> SYFEPTGPYLMVNVTGVDSKGNELLSPHYVEFPIKPGTTLTKEKIEYYVEWALDATAYKEFRVVELDPSAKIEVTY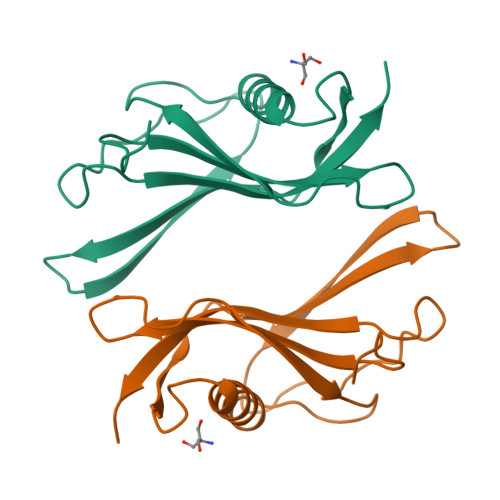YDKNKKKEETKSFPITEKGFVVPDLSEHIKNPGFNLITKVVIEKK> MDPMIIRGIRGARINNEIFNLGLKFQILNADVVATKKHVLHAINQAKTKKPIAKSFWMEILVRASGQRQIHEAIKIIGAKDGNVCLICEDEETFRKIYELIGGEIDDSVLEINEDKERLIREIFKI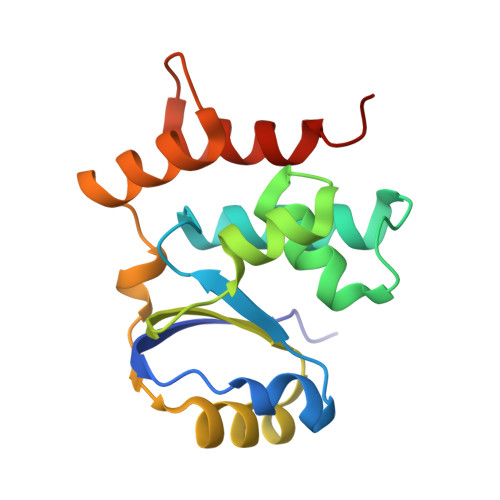RGFGNVVERVLEKIALIELKKE> MVRSFIYEAFQIPSGSMM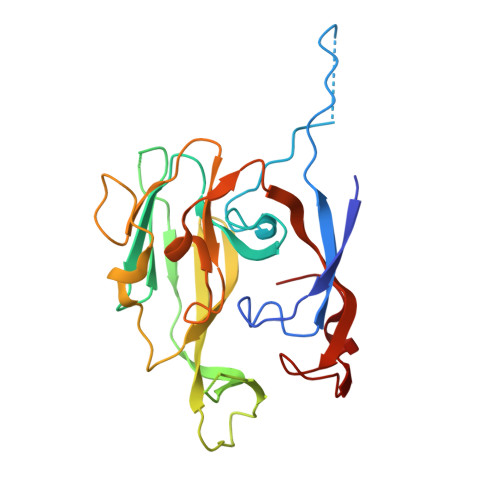PTLLIGDFILVEKFAYGIKDPIYQKTLIETGHPKRGDIVVFKYPEDPKLDYIKRAVGLPGDKVTYDPVSKELTIQPGCSSGQACENALPVTYSNVEPSDFVQTFSRRNGGEATSGFFEVPKNETKENGIRLSERKETLGDVTHRILTVPIAQDQVGMYYQQPGQQLATWIVPPGQYFMMGDNRDNSADSRYWGFVPEANLVGRATAIWMSFDKQEGEWPTGLRLSRIGGIH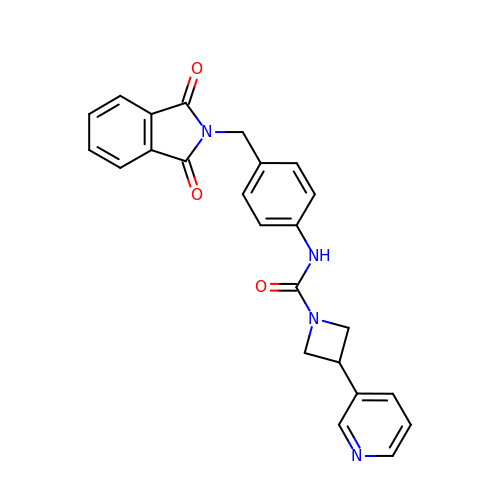N-{4-[(1,3-dioxo-1,3-dihydro-2H-isoindol-2-yl)methyl]phenyl}-3-(pyridin-3-yl)azetidine-1-carboxamide | C24 H20 N4 O3 | BXJQNJNBPGVHBT-UHFFFAOYSA-N> ALPDFTSDRYKDAYSRINAIVIEGEQEAHDNYIAIGTLLPDHVEELKRLAKMEMRHKKGFTACGKNLGVKADMDFAREFFAPLRDNFQTALGQGKTPTCLLIQALLIEAFAIS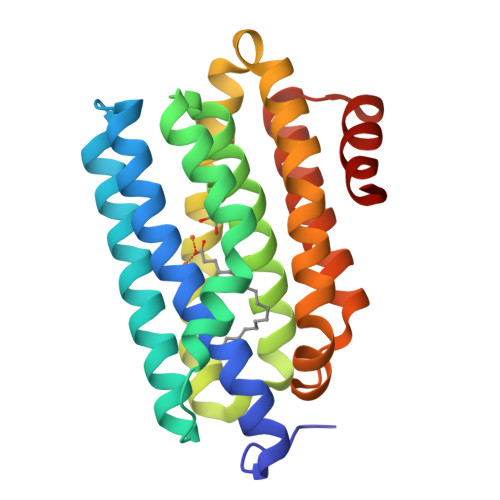AYHTYIPVSDPFARKITEGVVKDEYTHLNYGEAWLKANLESCREELLEANRENLPLIRRMLDQVAGDAAVLQMDKEDLIEDFLIAYQESLTEIGFNTREITRMAAAALVS>KLDAKAYFDEKLRELTAAVATIATSYLLAHVNQDQHVVMLTSCLPGEGKTTSSLNLALSLAQMEKTLLIDCDLRKPAIAHRFGISGSQPGVTNLLNGTQSLEDCVYHDEQSGLDILTAGVYASNPLELLSSSKFSELLADLRT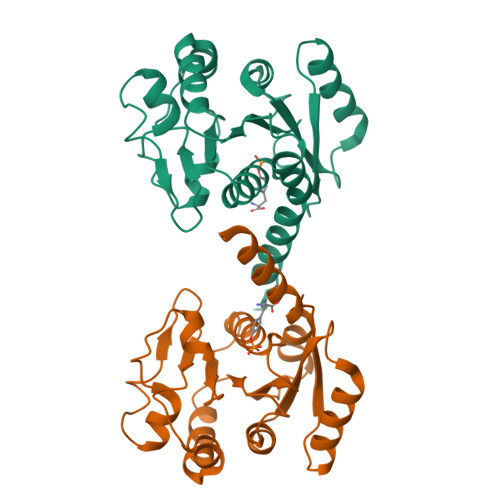RYQRIVIDTPPCLAVSDSFMLAQYVDSVILVIDANHTRTPVVREVVGKLTQQGSRIDGVILNRLNAKKASRYSGYYHYQAYYGEETKSGAAK[2x]ADENOSINE-5'-[PHENYLALANINOL-PHOSPHATE] | C19 H25 N6 O7 P 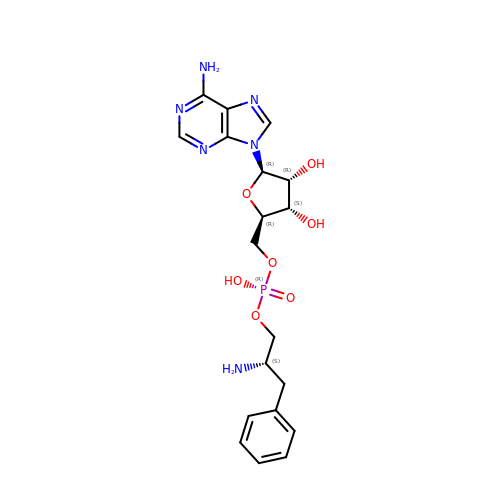| XNEAAYNJQROQFE-BPAMBQHCSA-N>MLNKVIKTTRLTAEDINGAWTIMPTPSTPDASDWRSTNTVDLDETARIVEELIAAGVNGILSMGTFGECATLTWEEKRDYVSTVVETIRGRVPYFCGTTALNTREVIRQTRELIDIGANGTMLGVPMWVKMDLPTAVQFYRDVAGAVPEAAIAIYANPEAFKFDFPRPFWAEMSKIPQVVTAKYLGIGMLDLDLKLAPNIRFLPHEDDYYAAARINPERITAFWSSGAMCGPATAIMLRDEVERAKSTGDWIKAKAISDDMRAADSTLFPRGDFSEFSKYNIGLEKARMDAAGWLKAGPCRPPYNLVPEDYLVGAQKSGKAWAALH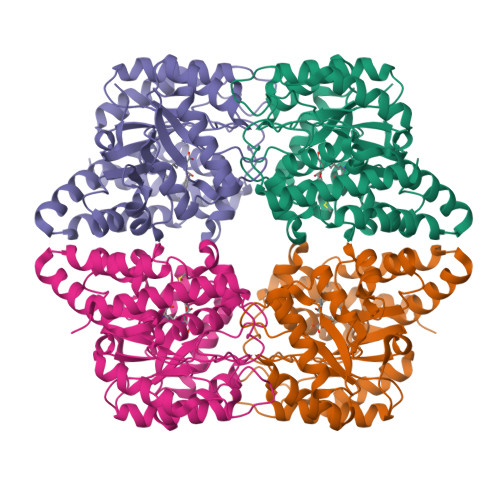AKYSK[2x]> MAVPFVEDWDLVQTLGEGAYGEVQLAVNRVTEEAVAVKIVDMKRAVDCPENIKKEICINKMLNHENVVKFYGHRREGNIQYLFLEYCSGGELFDRIEPDIGMPEPDAQRFFHQLMAGVVYLHGIGITHRDIKPENLLLDERDNLKISDFGLATVFRYNNRERLLNKMCGTLPYVAPELLKRREFHAEPVDVWSCGIVLTAMLAGELPWDQPSDSCQEYSDWKEKKTYLNP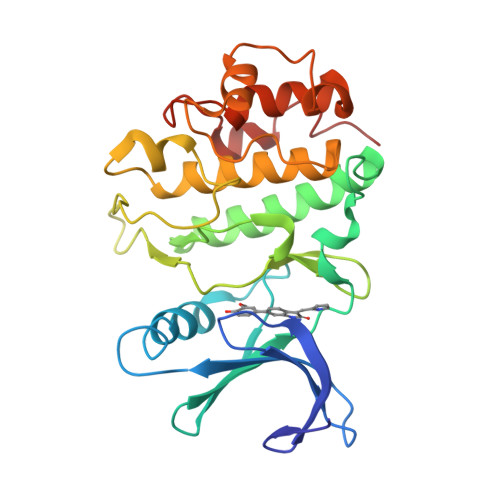WKKIDSAPLALLHKILVENPSARITIPDIKKDRWYNKPL>[4x]AEQSGKSQTVIVGPWGAQVSTS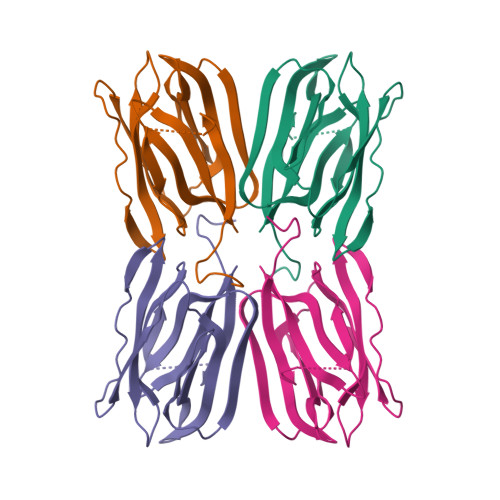SNGKAFDDGAFTGIREINLSYNKETAIGDFQVIYDLNGSPFVGQNHTSFITGFTPVKISLDFPSEYIIEVSGHTGKVSGYVVVRSLAFKTNKKTYGPYGVTSGTPFNLPIENGLIVGFKGSIGYWLDYFSMYLSL> RDFNNLTKGLCTINSWHIYGKDNAVRIGEDSDVLVTREPYVSCDPDECRFY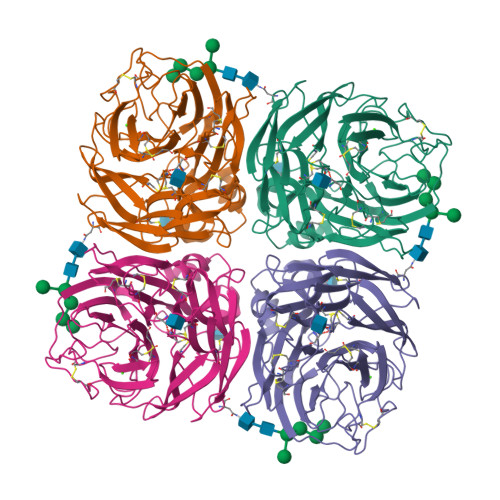ALSQGTTIRGKHSNGTIHDRSQYRALISWPLSSPPTVYNSRVECIGWSSTSCHDGKTRMSICISGPNNNASAVIWYNRRPVTEINTWARNILRTQESECVCHNGVCPVVFTDGSATGPAETRIYYFKEGKILKWEPLAGTAKHIEECSCYGERAEITCTCRDNWQGSNRPVIRIDPVAMTHTSQYICSPVLTDNPRPDDPTVGKCNDPYPGNNNNGVKGFSYLDGVNTWLGRTISIASRSGYEMLKVPNALTDDKSKPTQGQTIVLNTDWSGYSGSFMDYWAEGECYRACFYVELIRGRPKEDKVWWTSNSIVSMCSSTEFLGQWDWPDGAKIEYFL>[2x]MKAVLEQFGFPLTGTEARCYTNHALSYDQAKRVPRWVLEHISKSKIMGDADRKHCKFKPDPNIPPTFSAFNEDYVGSGWSRGHMAPAGNNKFSSKAMAETFYLSNIVPQDFDNNSGYWNRIEMYCRELTERFEDVWVVSGPLTLPQTRGDGKKIVSYQVIGEDNVAVPSHLYKVILARRSSVSTEPLALGAFVVPNEAIGFQPQLTEFQVSLQDLEKLSGLVFFPHLDRTSDI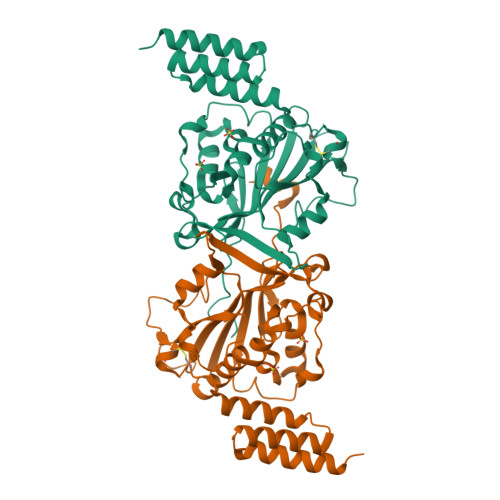RNICSVDTCKLLDFQEFTLYLSTRKIEGARSVLRLEKIMENLKNAEIEPDDYFMSRYEKKLEELKAKEQSGTQIRKPSHHHHHH> GSHMRSRRVDVMDVMNRLILAMDLMNRDDALRVTGEVREYIDTVKIGYPLVLSEGMDIIAEFRKRFGCRIIADFKVADIPETNEKICRATFKAGADAIIVHGFPGADS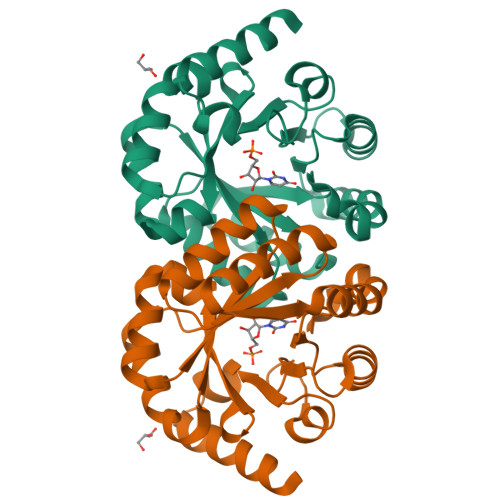VRACLNVAEEMGREVFLLTEMSHPGAEMFIQGAADEIARMGVDLGVKNYVGPSTRPERLSRLREIIGQDSFLISPGVGAQGGDPGETLRFADAIIVGRSIYLADNPAAAAAGIIESIKDLRIPEDPAANKARKEAELAAATAEQ>[4x]MINGIKNLFSYLFDSKDYSTFSGVVDIIVVRQPDDSLKSMPFHIRFGTLKVLDNQNINIQITVNDKKIEDVFMLMLPEGACYFPELNAKNEIQKKLRPSSAILKKFNLKNGYNKIQFIAESDLQGKQLIEGKIYLYNYDTKLVISDVDGTVTKSDVKGHISTIIGKEWTHDDIAELYTNIQKNGYKMVYLSSRPLYFYNYTQG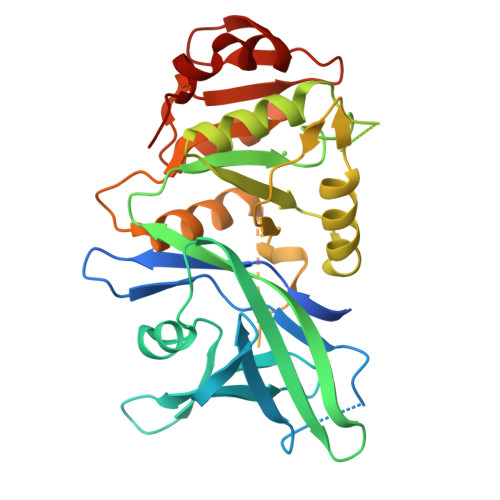YLKGIIQNGFTMPDGPILLSPDQIISSLNREVVYKKADEFKGALLKDLRRVFPEEVNPIFAGFGNRDTDATACLYAGVIIDNIFIINEQSQVEILGKQEKSSYKKINEKIQELFPRLP> MRVNNGLTPQELEAYGISDVHDIVYNPSYDLLYQEELDPSLTGYERGVLTNLGAVAVDTGIFTGRSPKDKYIVRDDTTRDTFWWADKGKGKNDNKPLSPETWQHLKGLVTRQLSGKRLFVVDAFCGANPDTRLSVRFITEVAWQAHFVKNMFIRPSDEELAGFKPDFIVMNGAKCTNPQWKEQGLNSENFVAFNLTERMQLIGGTWYGSEMCKGMFSMMNYLLPLKGIASMHCSANVGEKGDVAVFFGLSGTGKTTLSTDPKRRLIGDDEHGWDDDGVFNFEGGCYAKTIKLSKEAEPEIYNAIRRDALLENVTVREDGTIDFDDGSKTENTRVSYPIYHIDNIVKPVSKAGHATKVIFLTADAFGVLPPVSRLTAD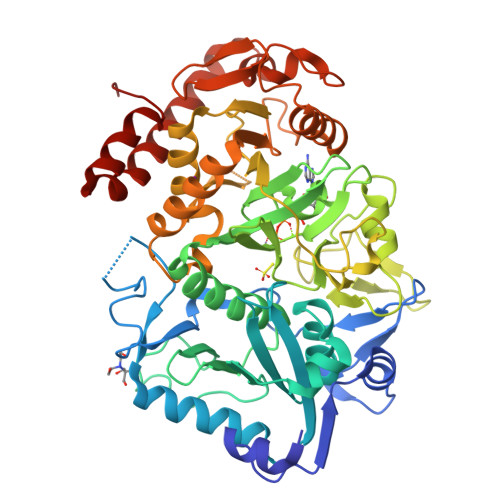QTQYHFLSGFTAKLAGTERGITEPTPTFSACFGAAFLSLHPTQYAEVLVKRMQAAGAQAYLVNTGWNGTGKRISIKDTRAIIDAILNGSLDNAETFTLPMFNLAIPTELPGVDTKILDPRNTYASPEQWQEKAETLAKLFIDNFDKYTDTPAGAALVAAGPKLHHHHHH>[4x]MTPDELNSAVVTFMANLNIDDSKANETASTVTDSIVHRSIKLLEVVVALKDYFLSENEVERKKALTCLTTILAKTPKDHLSKNECSVIFQFYQSKLDDQALAKEVLEGFAALAPMKYVSINEIAQLLRLLLDNYQQGQHLASTRLWPFKILRKIFDRFFVNGSSTEQVKRINDLFIETFLHVANGEKDPRNLLLSFALNKSITSSLQNVENFKEDLFDVLFCYFPITFKPPKHDPYKISNQDLKTALRSAITATPLFAEDAYSNLLDKLTASSPVVKNDTLLTLLECVRKFGGSSILENWTLLWNALKFEIMQNSEGNENTLLNPYNKDQQSDDVGQYTNYDACLKIINLMALQLYNFDKVSFEKFFTHVLDELKPNFKYEKDLKQTCQILSAIGSGNVEIFNKVISSTFPLFLINTSEVAKLKLLIMNFSFFVDSYIDLFGRTSKESLGTPVPNNKMAEYKDEIIMILSMALTRSSKAEVTIRTLSVIQFTKMIKMKGFLTPEEVSLIIQYFTEEILTDNNKNIYYACLEGLKTISEIYEDLVFEISLKKLLDLLPDCFEEKIRVNDEENIHIETILKIILDFTTSRHILVKESITFLATKLNRVAKISKSREYCFLLISTIYSLFNNNNQNENVLNEEDALALKNAIEPKLFEIITQESAIVSDNYNLTLLSNVLFFTNLKIPQAAHQEELDRYNELFISEGKIRILDTPNVLAISYAKILSALNKNCQFPQKFTVLFGTVQLLKKHAPRMTETEKLGYLELLLVLSNKFVSEKDVIGLFDWKDLSVINLEVMVWLTKGLIMQNSLESSEIAKKFIDLLSNEEIGSLVSKLFEVFVMDISSLKKFKGISWNNNVKILYKQKFFGDIFQTLVSNYKNTVDMTIKCNYLTALSLVLKHTPSQSVGPFINDLFPLLLQALDMPDPEVRVSALETLKDTTDKHHTLITEHVSTIVPLLLSLSLPHKYNSVSVRLIALQLLEMITTVVPLNYCLSYQDDVLSALIPVLSDKKRIIRKQCVDTRQVYYELGQIPFE

Here we report cryo-EM structures of the HEAT-repeat protein Met18 from Saccharomyces cerevisiae, a key component of the CIA targeting complex (CTC) that identifies cytosolic and nuclear client proteins and delivers a mature iron-sulfur cluster. Met18 is a 118 kDa alpha solenoid protein comprised entirely of HEAT (Huntingtin, elongation factor 3 (EF3) repeats, protein phosphatase 1A, and the yeast kinase TOR1) repeats. ScMet18 has a curved S-shaped structure comprised of 23 HEAT-repeat (HR) units; each HR contains two α-helices that are connected by loops. We find that in the absence of other CTC proteins, Met18 adopts tetrameric and hexameric states.

To address the preferred orientation issues that we observed with the Vitrobot-prepared cryo-EM grids, we prepared grids of ScMet18 (SUMO-tag was cleaved) using a chameleon, a commercially available piezoelectric cryo-EM plunger that is based on the SpotitOn plunger developed by Carragher and co-workers. To our surprise, the data collected from the chameleon sample had tetramers present in addition to the hexamers observed in the Vitrobot dataset. The tetramer contains 2-fold symmetry and was refined to 12.77 Å. Both the hexamer and the tetramer have similar overall dimensions and their chains have similar curvatures, despite the fact that the tetramer contains two fewer chains. As a result, the tetramer is less tightly packed than the hexamer, especially around the more exposed N-termini, since its protomers are shifted away from one another as compared to their relative orientation in the hexamer. The protomers of the tetrameric state appear to be less tightly packed than protomers of ScMet18 in the hexameric state, and thus the ScMet18 tetrameric state may be more prone to issues of particle denaturation. Notably, residues that appeared to be involved in binding Cia2 (R1010, R1013, R1020) are buried in both the hexameric and tetrameric states of ScMet18, indicating that ScCia2 cannot bind to ScMet18 without disrupting these higher order oligomeric states. Similarly, the N-terminal residues whose substitution was shown above to impair association with client protein ScLeu1 (R144, K187, F217) are partially buried in the hexamer and in two of the chains of the tetramer. In the other two chains of the tetramer, these N-terminal residues are mostly exposed.>SMKTIKVKNKTEGSKVAFRMLEEEITFGAKTLGLATGSTPLELYKEIRESHLDFSDMVSINLDEYVGLSADDKQSYAYFMKQNLFAAKPFKKSYLPNGLAADLAKETEYYDQILAQYPIDLQILGIGRNAHIGFNEPGTAFSSQTHLVDLTPSTIAANSRFFEKAEDVPKQAISMGLASIMSAKMILLMAFGEEKAEAVAAMVKGPV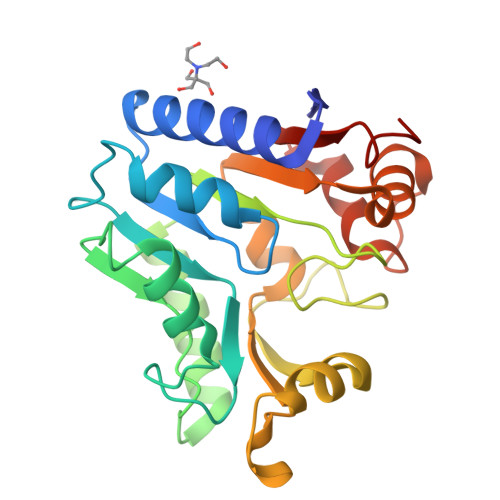TEEIPASILQTHPKVILIVDEKAGAGI[2x]> GMAIAPQQIQERLKQEQYQKFVVADIGNFPHCLAQTPEGIASGQRYQKYSTNSLSRTPPFSQWGAPQLLTPKSAQEYIKFAQQRNKKSSFKIDGEAVRVSECSNFAYHSAGVLLDDPQIRTQYDVAVIGSMHSNGR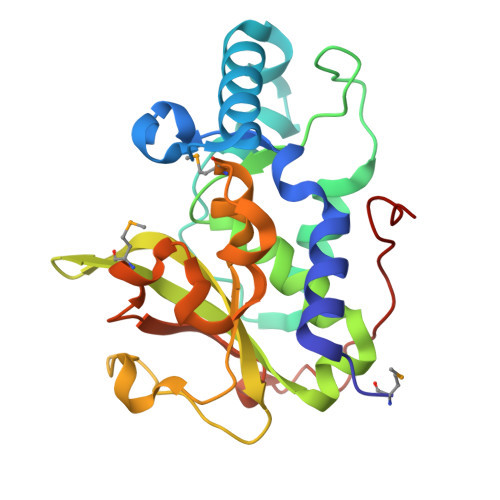YLHNITLLVPKGSRLPQPPQQLTAEVFPIGTLIVDPWAVGMGHPPEQALAIPKEQFAYNRSLFPATVNYQSALDESLTSTRTGQLTPYTGTPSRT2-(3-fluorophenyl)-N-{2-[2-(1H-imidazol-1-yl)pyrimidin-4-yl]ethyl}ethanamine 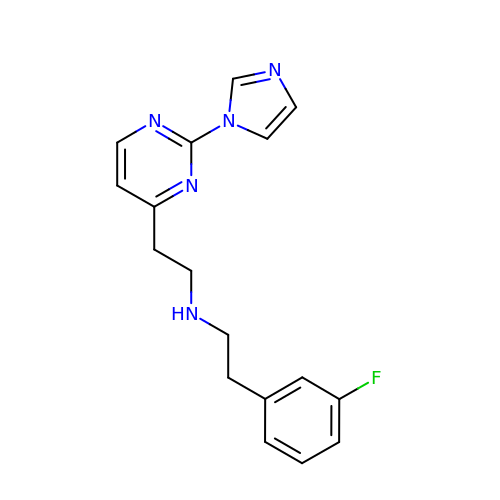| C17 H18 F N5 | ZPTNPJCYGBTULC-UHFFFAOYSA-N> MIINNKTPVGEVRPSQLLWTYGPGALIDLPSLSVVTLGIDRWERERCQPIQEARLLAAVRKVLGPQVENLRMPPFQKSELVDPWSAEANIGVPVRPFPRWMRCVKCGLLSPFDDGLLEIKEDRFRAERTRFVHKGCTGSKGNLPAKDADAVPARFLLACRDGHLDDFPWHYFVHGGNSTCKGTLRFFESGASLQTENLWVRCDSCEASRSMAHAFGKAGKENLPACRGRHPHLDQFDIDCGEEPRAVLLGATNSWFPITLSALAIPQSKNPLSQLIQDGWPLFEAITAEVMVPIVVQTLKLTGGLPGIDKYSVSDIWSAIEMHRSGGDSEFVGEADIKGPEWEVLTEANPPTDYPHFMSKKIGTPAQFIPYISRVLLLERLREVNALLGFTRVEAPEGSGEINERPQMASLARNKPEWVPANQVHGEGIFIQFNEKTLVAWESLDAVKQVDEMLRGGHTGWRNSRNLDPNEDYPGIRYAMLHTLSHL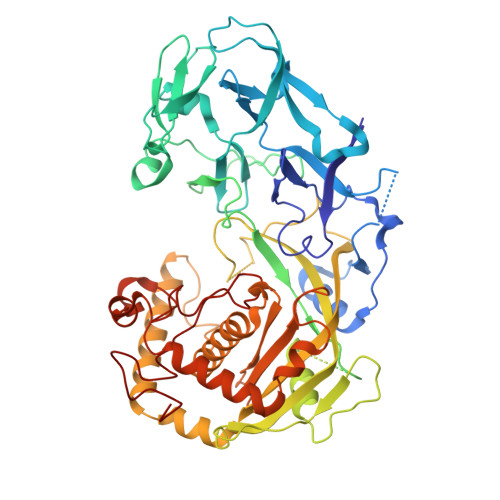LIRELALECGYNAASIRERIYADTSNGSPQAGILIYTAAADSDGTLGGLVDLGKPENLGRLLVQALNRSKICSSDPLCSEHNPEKDRSLHAAACHACTLVAETSCEQGNRYLDRSLLIPTLERIHAAFFKGF>[2x]GSHMGSRITYVKGDLFACPKTDSLAHCISED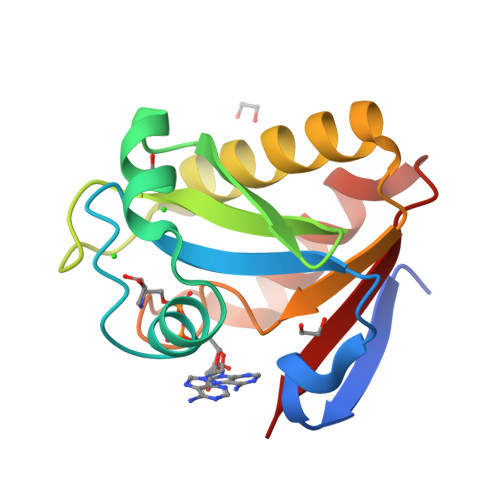CRMGAGIAVLFKKKFGGVQELLNQQKKSGEVAVLKRDGRYIYYLITKKRASHKPTYENLQKSLEAMKSHCLKNGVTDLSMPRIGCGLDRLQWENVSAMIEEVFEATDIKITVYTL>[2x]MEEPEEPADSGQSLVPVYIYSPEYVSMCDSLAKIPKRASMVHSLIEAYALHKQMRIVKPKVASMEEMATFHTDAYLQHLQKVSQEGDDDHPDSIEYGLGYDCPATEGIFDYAAAIGG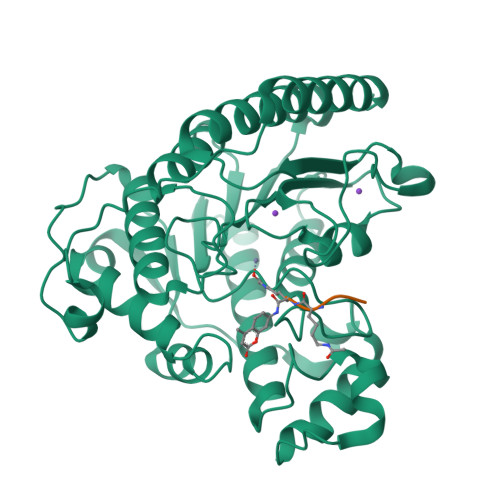ATITAAQCLIDGMCKVAINWSGGWHHAKKDEASGFCYLNDAVLGILRLRRKFERILYVDLDLHHGDGVEDAFSFTSKVMTVSLHKFSPGFFPGTGDVSDVGLGKGRYYSVNVPIQDGIQDEKYYQICESVLKEVYQAFNPKAVVLQLGADTIAGDPMCSFNMTPVGIGKCLKYILQWQLATLILGGGGFNLANTARCWTYLTGVILGKTLSSEIPDHEFFTAYGPDYVLEITPSCRPDRNEPHRIQQILNYIKGNLKHVVIEGRSHHHHHH;> GGG3-[3-(3-methyl-6-{[(1S)-1-phenylethyl]amino}-1H-pyrazolo[4,3-c]pyridin-1-yl)phenyl]propanamide | C24 H25 N5 O | 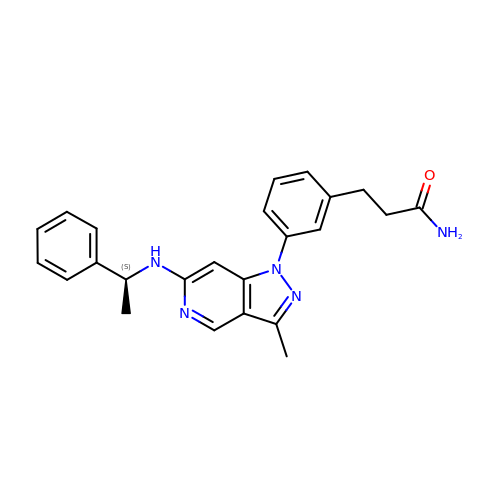ZFGCLYUGFRNYFE-INIZCTEOSA-N> QLSCTGPP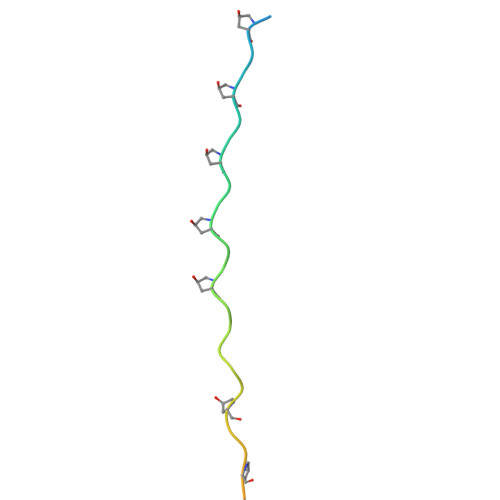AIPGIPGIPGTPGPDGQPGTPGIKGEKGLPGLAGDH>[3x]ATAAEIAALPRQKVELVDPPFVHAHSQVAEGGPKVVEFTMVIEEKKIVIDDAGTE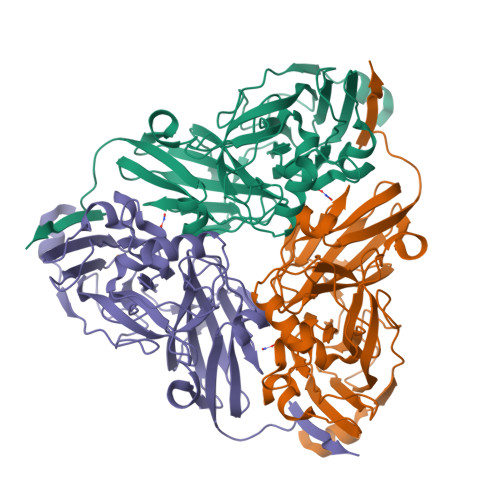VHAMAFNGTVPGPLMVVHQDDYLELTLINPETNTLMHNIDFHAATGALGGGGLTEINPGEKTILRFKATKPGVFVYHCAPPGMVPWHVVSGMNGAIMVLPREGLHDGKGKALTYDKIYYVGEQDFYVPRDENGKYKKYEAPGDAYEDTVKVMRTLTPTHVVFNGAVGALTGDKAMTAAVGEKVLIVHSQANRDTRPHLMGGHGDYVWATGKFNTPPDVDQETWFIPGGAAGAAFYTFQQPGIYAYVNHNLIEAFELGAAAHFKVTGEWNDDLMTSVLAPSGTIEGR>[3x]GGSSGVRLWATRQAMLGQVHEVPEGWLIFVAEQCELYVRCQNGFRKVQLEARTPLPR

We describe the development of a biologic that takes advantage of the proximity of the N-terminus of bound ACE2 to the three-fold symmetry axis of the spike protein to create an ultrapotent, trivalent ACE2 entry antagonist. Therefore, we sought trimeric scaffolds to fuse three ACE2 moieties and leverage the inherent symmetry of the spike trimer to maximize avidity. Thus, we determined a trimeric antagonist fused to the N-terminus of ACE2 would require a short peptide linker and would be less likely to form inter-spike interactions. The collagen VIII trimerization domain is significantly larger than the collagen XVIII domain (44.7 kDa and 19.3 kDa, respectively), but more importantly, previous studies reported that collagen VIII melts at ~45 °C66, whereas the collagen XVIII domain melts at ~85 °C (vide infra). Given these observations, the smaller, more thermally stable collagen XVIII trimerization domain was advanced to develop the trimeric antagonist.

We then sought to prevent the dissociation of the collagen XVIII trimer via the introduction of intermolecular disulfide bonds, despite the high reported trimerization constant (where 50% of the trimer is monomeric) of 56 pM49. Cysteine mutations capable of creating inter-chain disulfide associations (i.e., C®-C® distances less than 6 Å and absence of obvious steric clashes) were identified: G22–F'26, E31–V'37, and G(-1)–L’5. The parental construct yielded ~1.7 mg·L−1 purified protein (n = 1); the disulfide mutants, E31C–V'37C and G(-1)C–L’5C constructs, yielded each ~1 mg·L−1 protein each (n = 1); whereas the G22C–F'26C mutant only yielded ~0.05–0.2 mg·L−1 protein (n = 2). The formation of inter-chain disulfide bonds was confirmed by X-ray diffraction studies. High-resolution crystal structures of the E31C–V'37C and G(-1)C–L’5C mutants afforded clear electron density for the disulfide bonds in both mutants (respectively). Furthermore, the thermal stability of each collagen disulfide mutant was assessed by DSF. The ‘wildtype’ collagen XVIII trimerization domain produced a calculated melting temperature of 84.9 ± 0.2 °C. However, two of the disulfide mutants (G(-1)C–L’5C and E31C–V'37C) either produced very low or no fluorescent intensity up to 100 °C. Considering the high melting temperature of the “parental” collagen XVIII, we posit that the melting temperatures of the disulfide mutants exceed 100 °C. Given the poor expression of the G22C–F'26C mutant with our trimeric ACE2 constructs, we proceeded with E31C–V'37C. The introduction of E31C–V'37C to the trimerization domain of T3A (termed TD3A) afforded a melting temperature of 51.1 ± 0.03 °C. Combining the disulfide mutations, TD3A with T3AD (termed TD3AD), further increased the melting temperature to 56.5 ± 0.01 °C.> MPITIHAPLPPPRLHDEDSDVDMSSDSDSSSEGGVPLTSNLPSRAKPKSSLFTTTKSSSDIVTPGELITTSPQFMRGHGTYIPPGTTSIISSVAGTILRTNKLLSVRPLRARY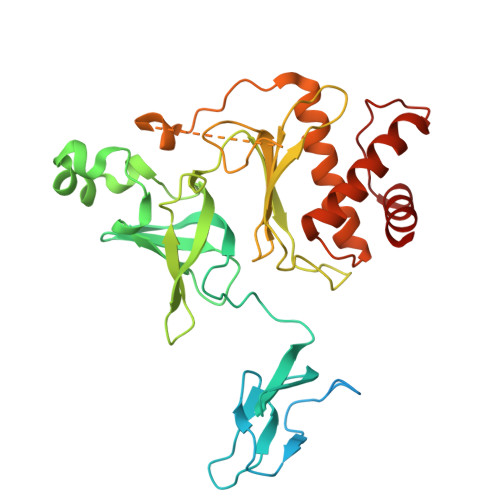TPEVGDLVVGRIIEVQARRWRVDVGSTQFASLPLSAINLPGGILRKRTETDELQMRSFFSEGDLLVAEVQGVYGDGGAVLHTRSLKYGKLRNGVFVAVSGMGGGGGVVRSRRQVWTLEGANGAGLIDVVLGVNGYVWIAKHTEDGPGEDPNASTKQVGITNLEEGMSANMYSSQNDRIEAETMREIARLRGVVMALVENGLRVDEDMVMRGYREAVEMALVSPEGPEDVYLGGERGRQLAAALTA> 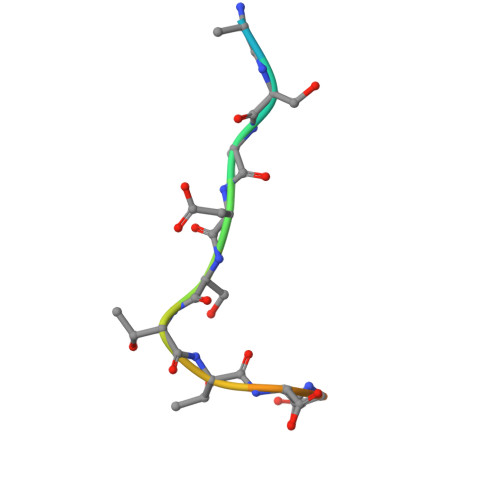KAASADSTTEGTPAD>[4x]HHHHHHMPDSYVHRHVVTFDETNLVGNVYFAHYLHWQGHCREHFLADHAPGVMAALADGLALVTVDCHADFYAEGSAFDEV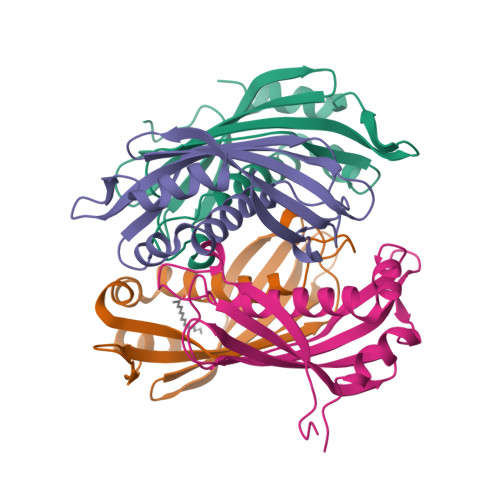EVRMMLDRLDGHRIAMSFDYVRVAPGPPTLLAQGRQTVACMRRAGHGLEPVEVPAELRRALSRYAVVAR>[2x]EEVRQFRRLFAQLAGDDMEVSATELMNILNKVVTRHPDLKTDGFGIDTCRSMVAVMDSDTTGKLGFEEFKYLWNNIKKWQAIYKQFDV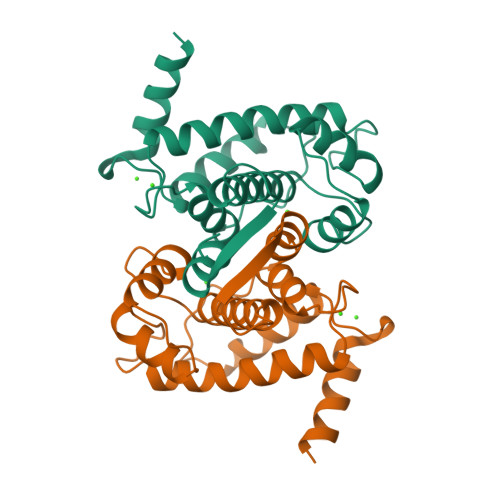DRSGTIGSSELPGAFEAAGFHLNEHLYSMIIRRYSDEGGNMDFDNFISCLVRLDAMFRAFKSLDKDGTGQIQVNIQEWLQLTMYS>MISDLACLDAKDIVELMRFLPHRYPFLLVDKVVNIQRDESAIGIKNVTFNEPHFMGHFPGRPVMPGVLILEGMAQTAGAICAIHNGFDQYAPPYLMSIDKARFRKPVFPGDRLEYHVNKVRNRVDLWKFQCCAKVENTVVAEAEICAMVMHEKKEKN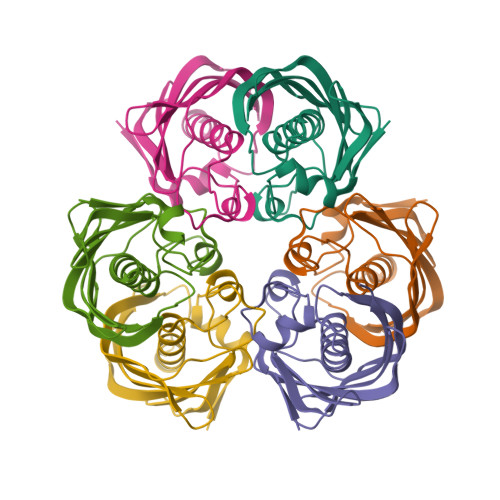ESHG[3x]> MGRKKIQITRIMDERNRQ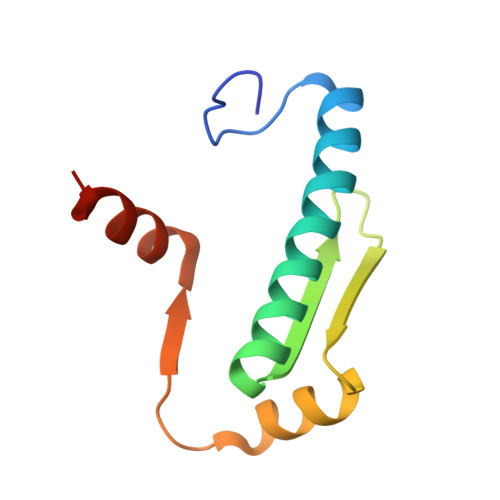VTFTKRKFGLMKKAYELSVLCDCEIALIIFNSSNKLFQYASTDMDKVLLKYTEYSEPHESRTNTDILETLKRREHRG> MSTIEERVKKIIGEQLGVKQEEVTNNASFVEDLGADSLDTVELVMALEEEFDTEIPDEEAE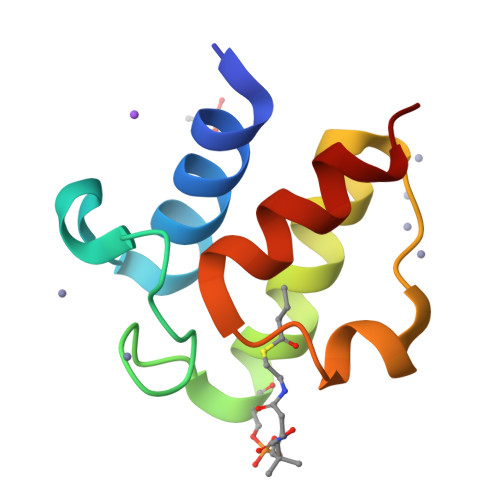KMTTVQAAIDYINGHQA>[2x]VAFGADAAKTTQEKFDALKEAGVFSGYPGTTDAKLGQDM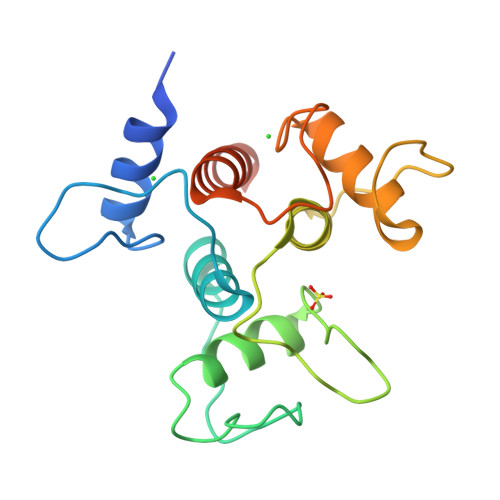TRAEFAKVLVKLFGLKEIHGQYSYKDKNYDAKNWAAPFIEAVTAEGLMQGKDLTKKIFDFNGKITVEEASKTLVTALKLEPVKDAQNKATDWAKGYFEAAVNAGLFSKDANPKANATRAQLVEAAFAADEMSKGSGSHHHHHH>[2x]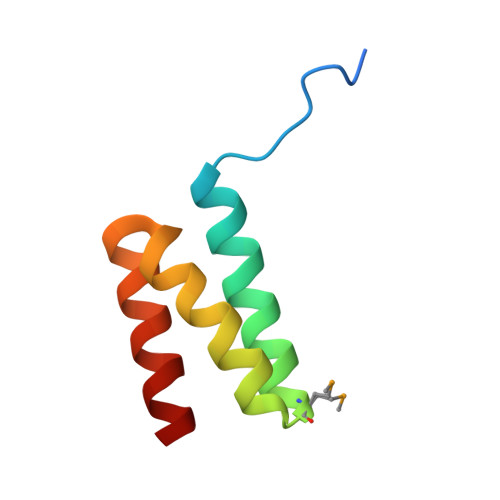GIDPFTDDFDFLSGADEAATKLDLARAYIDMGDSEGARDILDEVLAEGNDSQQAEARELLERLA> MSSTHIEQ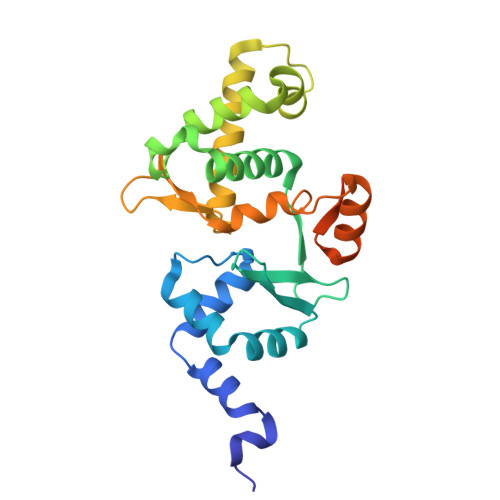FMPVKLAQALANSLFPELDSQLRAGRHIGIDDLDNHAFLMDFQEQLEEFYARYNVELIRAPEGFFYLRPRSTTLIPRSVLSELDMMVGKILCYLYLSPERLANQGIFTSQELYEELISLADEGKLMKFVNQRSSGSDLDKQKLQEKVRTTLNRLRRLGMVYFLPNNNNKFTITEAVFRFGADVRSGDDPREIQLRMIRDGEAMPVEGSLSLDDSENDETPDNSAEGAGDEQP>MSLSPHVENASIPKGSTPIPKNRNVSSIGKGEFLGSSSSNNSSFRMNHYSNSGQPSVLDSIRRPNLTPTFSYSNGVYMPESHRTSSFNDSYLPYDKNPYAKTTGSMSNKSNMKIKTKKNAINTNTRKSSGLIYTTKVDKELSSIDKVNDPNINGLVCAGKTHLGLYKFSPSDRSIKCVHDFITPNSNTSTRGTTSLLPKLSKRTRQNKFSTIADVKTGFNNYKNCIAVCNNSTAISIYDLNKSSSIDNPLITSLCEHTRSINSFDFNMVESNLIISGGQDSCVKIWDLRSNKSKSSNRSDISINTASDSIRDVKWMPGYNFASKNDQGSSTYGNLKSGYKFASIHDSGYLLKFDLRQPAQYEKKLNAHTGPGLCLNWHPNQEYIATGGRDGKCCLWFVGDNANAAENTVLNYGNSPSLHAPNTSLNNSGSLAFPKLTINTGYPVTKLKFKPAYSSNIYNSLLGISSMGDEAEVRIYSLARKYIPKHVLLSETPSLGLVWWDENLIFNIDKGTRINGWDINKEPTVLENLSKNTTTWRDLDGNGLLSVDQEIGSYEVVEPELQPTSSTTCKKHPGTIKNPKNGNPENQGIIGGIKKGFSHTGLTSFTPERPPTLKAGPTFSTKSLTLASGASSFNSSSASLTSLTPQTENREEIAIEPPCIITLDIPQIFNNIRLTKIAHSRKKNVISESSSMKNSPVEKFKYLARQLKFSYIREHNVSDSADTAYKNDIENIDVVKNATETHGDNTTTTNNNDDGDDDDDDDDDDKIIESHLLKKYNFPENNTWATLMNEKVNNKKSKRNSSSSREFDEKDVRSSISSISASRQSHDRARKIDKNVEAELQEKIQTLVDLISIATHNASVYLSIDDLTNFKIWILIRDSLLWDLKWMTSSQISSDNASNMDANESSDFEAGENLKTGKEFPEEDGAGTSGAESLVEERPQAFRANSDEPSDAEKKPVSKLKEQLKNTEIIPYAQPNEDSDEVLTKLKELQNQRLESRTKMGETVSDDVIIEEDEHEHQEEEQPHDSPTKSAQFHASPIAKSIPILQKREHRKSFIDTFMLHSPNGYNGDTDIGNEDDNISPRFTYNSVSPRSKVSSLQSYATTTSQLETFKKLSSHTAPIIGSPRHAPSRPDSIGREQLSSSLTKKLAKCKKIIADPPWDTKKLIKQLYNQATETGNVVLTVNILFLFQTIYQITEIDIAKDAIAHFLLLLHRYELFGIAADVLKYCPFEDIMGSEGDQSSIRLFCERCGELITNESSKEKLRAEAQQTGNKKIMDKFGYWYCDSCKKKNTSCVLCERPLKKLTMVILPCGHEGHFQCIQEWFLDENEQECPGGCPGVAFI[2x];>[4x]MGLIKKVTHWSYDNLIDYLSVNPTRDEVTHYKVDPENESDESIIKLHTVKDFGSITCLDYSESEIGMIGVGEKNGYLRIFNISGQNSSSPASHAPVGLNANNETSMTNASGGKAAQAENIVGSVSNLKDTQGYPVSETNYDIRVRAKKQRCINSLGINTNGLIAMGLDRNKHDSSLQIWDMNYHDDSHETINPMFSYCTNESIVSLKFLNDTSVLAASTKFLKEIDVRSPNPIYQHPTRLTYDIKLNPFNDWQFSTYGDDGTLAIWDRRKLSDQASLGDLNVASPLLTFEKLVGSGAASRKYMNSCFRWSCVRNNEFATLHRGDTIKRWRLGYYCDSNRDIAADDDNEMNIENLFVSSVHDTNTMYDRVATFDYIPRSNNGTSLICMRQSGTIYRMPISEVCSKAILNNRNSLLLSNFENTEIDEIRVNNEHEKSNLENVKTILKNLSFEDLDVSEDYFPSGHDEPNNEIEYSELSEEENEGSNDVLDSKRGFELFWKPEKLLEKDISVIMRTRASLGYGLDPMNTVEMIDSSKNLQNNAYIRNTWRWIAIAKASVDDGTMVSGDLDLGYEGVIGIWNGINGISNQDRYRQETILSDKQLNKEMEKIIKLRRKNRDRNSPIANAAGSPKYVQRRLCLIISGWDLSRSDYEDKYNIIMKNGHYEKAAAWAVFFGDIPKAVEILGSAKKERLRLIATAIAGYLAYKDLPGNNAWRQQCRKMSSELDDPYLRVIFAFIADNDWWDILYEPAISLRERLGVALRFLNDTDLTTFLDRTSSTVIENGELEGLILTGITPNGIDLLQSYVNKTSDVQSAALISIFGSPRYFRDQRVDEWIQTYRDMLKSWELFSMRARFDVLRSKLSRTKTGVLTADIKPRQIYIQCQNCKQNINTPRTSSPSSAVSTSAGNYKNGEAYRRNNADYKKFNTGSSEAQAADEKPRHKYCCPHCGSSFPRCAICLMPLGTSNLPFVINGTQSRDPMQTEDSQDGANRELVSRKLKLNEWFSFCLSCNHGMHAGHAEEWFDRHNVCPTPGCTCQCNK;>MCSSINEGPYNSPTFGKSLSLKVDGGFNAVSINPSGRDIVLASRQGLYIIDLDDPFTPPRWLHHITPWQVADVQWSPHPAKPYWIVSTSNQKAIIWNLAKSSSNAIEFVLHGHSRAITDINFNPQHPDVLATCSVDTYVHAWDMRSPHRPFYSTSSWRSAASQVKWNYKDPNVLASSHGNDIFVWDLRKGSTPLCSLKGHVSSVNSIDFNRFKYSEIMSSSNDGTVKFWDYSKSTTESKRTVTTNFPIWRGRYLPFGEGYCIMPMVGGNNAVYLINLCDDDDSEQNKKTKLQPIYAFKGHSDRVIDFLWRSRHTCDGDYDDREFQLVTWSKDCDLKLWPISDSIYGKVNFDRGKRLEEKLPDYDYCSYNKEPENRENVQKNEFRRLRENFVTTSGLKKNKTNHITWLSGIRMNSATSQEDLFNETKIQNLGEEVSAIGHKFPKVVFEKISVSTRELCLTLNGPWSEENPDDYIFLRISINFPLNYPNKGDPPKFTIEENSNLTMSKRQEILSNLATIGQKYTDSNLYCLEPCIRFVLGEKVSLEDIEEGQEPLLNFDIADHIDFEELSSLDSSYSDSQNPENLSSQSDIESYKEALVFPDTSNQGLDFGRNLALDTTPVPNGCGSCWTATGELFCFFANEKKPEKKQNAIIKLSQKEAGVEKHPFKIEPQVLYDKEVDSSVITAADELKARPKRYVDTLGLGGGTNGDSRTYFDDETSSDDSFDSVADDWDDILRNDIIVRTKIPILRGNFKAFSSVHSESGKTVESTKKNKNLVISKNFSSLLSDRKELALEYLFMDATPEGFARNNALVAEKFDLDEISHCWQILSDMLIDQSDYDPYTTIWNNHPMGIKWFIKEAIVYFERQQNLQMLAMLCCVILSARRKKIPARYYGQELENMEGTIVFNDNESQNTSFWKGSDAFSTRSRSSTVTPNFYGNHLRGKNIHGGDNSSIRSDDHHARLRTHNTLNGSSKFTEPAQKQGSRAISSSPFHSRMPDIKVELLHDDIIEAYEQEDLLHLEVSDIPKFQTYIYQYSKLLFRWGLPLERVKILKVSTDFRSSYSSQGIPPNNNKKSPYNGVLTHWIENNEFGEEKFLARNCNYCDLRVTRSSFICGNCQHVLHSSCARIWWEIGDECPSGCGCNCPEMFDA[2x];>[6x]MQPFDSGHDDLVHDVVYDFYGRHVATCSSDQHIKVFKLDKDTSNWELSDSWRAHDSSIVAIDWASPEYGRIIASASYDKTVKLWEEDPDQEECSGRRWNKLCTLNDSKGSLYSVKFAPAHLGLKLACLGNDGILRLYDALEPSDLRSWTLTSEMKVLSIPPANHLQSDFCLSWCPSRFSPEKLAVSALEQAIIYQRGKDGKLHVAAKLPGHKSLIRSISWAPSIGRWYQLIATGCKDGRIRIFKITEKLSPLASEESLTNSNMFDNSADVDMDAQGRSDSNTEEKAELQSNLQVELLSEHDDHNGEVWSVSWNLTGTILSSAGDDGKVRLWKATYSNEFKCMSVITAQQ;>[2x]MVVIANAHNELIHDAVLDYYGKRLATCSSDKTIKIFEVEGETHKLIDTLTGHEGPVWRVDWAHPKFGTILASCSYDGKVLIWKEENGRWSQIAVHAVHSASVNSVQWAPHEYGPLLLVASSDGKVSVVEFKENGTTSPIIIDAHAIGVNSASWAPATIEEDGEHNGTKESRKFVTGGADNLVKIWKYNSDAQTYVLESTLEGHSDWVRDVAWSPTVLLRSYLASVSQDRTCIIWTQDNEQGPWKKTLLKEEKFPDVLWRASWSLSGNVLALSGGDNKVTLWKENLEGKWEPAGEVHQ;>[2x]MLSYFQGFVPIHTIFYSVFHPTEGSKIKYEFPPNNLKNHGINFNTFKNYIIPKPILCHKLITFKYGTYRIVCYPVTINSPIYARNFFSFNFVFVFPYDCETSPYEPAITRLGKMFKVLEEQNQLLSKSERDPVFFDLKVLENSTTTPSTAGPSSTPNPSSNTTPTHPTSEKDTKDMRSSRYSDLIKDLGLPQSAFSIQDLLMRIFQDLNNYSECLIPIDEGNAVDIKIFPLLRPPTTCVSLEDVPLSSVNLKKIIDVNWDPTMMSIVPYIDGLNSIAKISKLSNSDPGLVIECIRHLIYYKCVTLSDIFQFSNIYAPSSLIRNFLTDPLMASDCQSYVTFPEVSKISNLPLNKSLGSGDQDSPSFSVRRKSKSSSIPSNPDSRTTSFSSTSRVSQNSSLNSSFSSIYKDWRQSQTSCSSSNIHVINNRNRFLPTRSCLFDLYRSLSQGQTLKTWYESKYMILKENNIDIRRFITFGLEKRIIYRCYSFPVMINAGSREPKEMTPIITKDLVNNDKLLEKRNHNHLLSATGSRNTAQSGNLKPERPSKVSFEMQRVSSLATGKSTMPKLSDEEEGILEESIRNAETFDKICVLLSKPKLEVESYLNELGEFKVINS;>MDECLPNSCLLGVHLVISTHSGPQIVYHYPPSNTAFLTNNPTKHQHLYGNHANLNKNTSTNKEEKLFNSGSTKTASQIALNESAKSYNTAITPSMTNTNTNNVTLPPTRSHANTVGSQSSIPAATNGVGYRKTDIEDTSRTFQYQETESETSSSGLSDSELSTDYLDISSDSFSISSSLSSSSLSSSPSSSSSSSPPQDGLSRTNSSFQSTDSMSPTSPQMIMENDSISVAESYLDSGTNNKSRAASKRSQNFFHKLSTKKSTDSKTHSPVRKLKSKPSQSTKKGNKLLKNTSNETDGNAFTGSCSISSKKSLSSTGEHNQELRNSSLNDTPGQSPHHYHHRYHHYHKNAATSQRNSHTQYDVEEEDMEVSAMLQDGKISMNEIFFEEENFQDINKILEFDNDFVAEFCSPEREMCNTRFEFTVDNFCFLGLPIHVDSQGRWRKSKHKNKTRSKRSSSTTTNISRKKSIASKISSLSENTLKKVNSGEADTVYDSNIGHEASTDTPNLRINTDVSGNEFEREKEDLGKNMNMFHVCFVMNPHLIEYNKRIDDMYQFVVTRLSLLLRYVQSKTSYISSECHIILKEKERVLKHSKTYQSIRGAGNKGKYLYQRILAKSSLARALTECVDKIQRNEIACLEINDDKVISLQIPIQNEFEKMPNFKLQPVLRGSYLTSILNMKFLEKSSLRIESQNRQNDQAQFSDTNNNIYRFGNNINSTGHCGAANVDDGDDNESNYYCDDNDDLLNYALLLLDEPNNIISSLETFSYQDDIGTIILKHLVRNIQPNIPLRSYRYLITDLLDNPSSLDDLTTETNSLESSILRSCALHLMYWRHARIVIPLSSKYTYIVSPLAPIQGYTIDDYKSTSQNDGNVKKMDDRENNKSGSDRVPLIYQNSMLFRSKFPSLPSLPIFLSLLSTDKPQAYSNIIPSREHKPVYLNALAWLIQYGYVTQLLTFINIRVDKHIKMAVDEDLEKEGFRKTNTARRPSMDYKKTDKKLDDEDGQSRDANASEACSGKNEGMQSNDNNKDVDEKDNENDSRVDDRDDNEIAIADEEEILHFEYDDPEMQHDYTIILEPERATAIEKRWLYRCIYGQPSDIQILFNKLLKYFNGKVPMELVIIKEEISRHDLKKLLNALDKYLIEIHHW[2x];>MFAKLHGKKQRPISSINSQTPRTSNTTHANSISLSSGNLIVGSNRNLRQKKEQFGSQQRASGRKLISNKENDDNVNNGGDNNYDNGERVHRHHIPGLKIKAYQAELGYHESRFSENLVMLNLVEFPDIKPGDLVELKTYHKNPSASNGDKKIYFIAKDFDGETKRRAKTSNVSILSGQLQTLLDLPSRSRIWIKLKPNKFDLQADVVEFNIKDCLLNRGDMWVLSSKLVDTCVFMDQRLAFLDSIRGTIKGIYRNGKKIVSGYIGEQTRIIFRSESARLIFLIQITDEMWNFEETGEQLFQKMVNSFFPKIFKKWKDVDTHHTITIAFAISMDLSDTSFKDLTPGESLKNSQDYFRIVVDQVSIIHWVDIMETLREEFMEIRKDLLNKQTDKGYSVANGRFSPVIKSNFLELVNFATTILTDPFKQLDLRHTTTHVMIISPGSGLFDVDYSLLRLTGKKLLSLEMTMDLICLSKAPLHIVPLFRYRDFENKLHHCVPLWLSVFFWNDHDKKSNSEWTPRCKIYDLQMMGITENELIREVDVEYLQLNKKVKSLSEFMNDYDKNAFEVKILCAGSNTKQSKKLNSKFDTVFENDVVVKARKIPATATTTHGNTKFIWRGPKVALPAIKDIQKPNVIPDLSIKTIEASFYDDCNTTNDKISTPTTSNNDNLEMNDSLVSVRSADNQNTSLALDSLKGLSKRNSLKDFTQRVITKFISNIDTSKNKKIKSTLLRDDVDNSPLGSNTPLPSSESKISGLKLQQKGLADENVISKRGNLIIKKNLSIFGLPSNEIMSGSPSSYLGSSHTRTSSKLSNMSDKAAFITEGQKSKHDDSNTYSLTQQLKHRISETWVDIKSPSIPVSSEFANELLPIRWKDVWPKYVARKYSKWRSFTTPAELPITISDFPSKDDFDRNFIFRNHSVTLNTDQEQYNQTYKDLLRDMIYMRLLTGFQICVGRQVEKIELSRESGESETVVNKYLDFNQNDAFKLYLMIDSEIHRITCSSSGIIDVERYLRKDEANLFDQVPSYIPLVKTRYESSFRDAMIDPLHVKRESLNWNQIDQVLAGYGDNLIDRKWHGFRAKYVVLPTDIPPNTYSMVINGKSETLNPEEIRVEGLRRLIGSITRSRLRTEKEKKGRKTKREEIQPEVMFYTGPLYNFINEQQTSLESSAINFKDSIFVNDNNLLNRNVELSKLAYQIQRGEDRITLVNRKWHWKKHEKCFVGSEMVNWLIRNFSDIDTREDAIKYGQKVMKEGLFVHVLNKHNFLDGHYFYQFSPEYVMDTNKLEKTNSHRSTLSDPKQMLRKASTGSSNDPSAMTPFSSVVPAISASNASVADAKEPSRPILMLSNSLVIDVDPAGKSSKQESCTVHYDRVHNPDHCFHIRLEWLTTTPKLIDDLVGNWSRLCERYGLKMIEIPWEELCTIPSVNPFHSFVEIKLAINPWEDPEFKDRELFAKSKFYYHVYLLKASGFLLDNRASKFLQNQDIEFDIMYSWG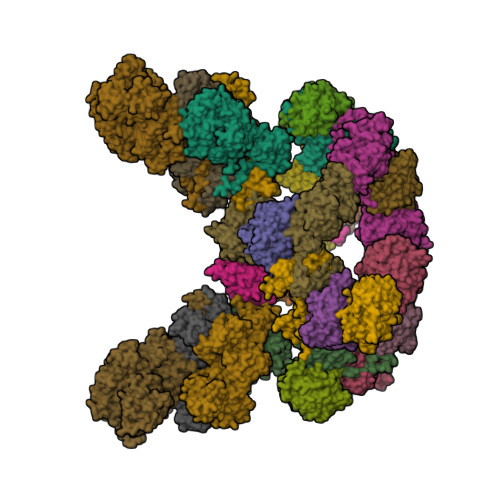KPQFKYVQYIHHTGAYVAELRENGCLFLAPNNIYISRVNPGNIIGKIHSASSSSLDAQKVILNFKSTCLDYQKLRSIFLDAKEMWITGKIVED[2x]The large terminase protein is a key component of the DNA packaging machinery in tailed bacteriophages and evolutionarily related herpes viruses. Typically, in addition to an ATPase domain which powers DNA translocation, the large terminase contains a nuclease domain which cuts concatemeric DNA, generated by rolling circle replication. Crystal structures of the large terminase nuclease from the thermophilic bacteriophage G20c show that it is most similar to the RuvC family of the RNase H-like endonucleases. The overall structure adopts the RNase-H fold.

Structures for complexes with Mn2+, Mg2+, Co2+ and Ca2+ were determined by soaking crystals of the apo protein, whereas the structure of the Zn2+ complex was obtained by co-crystallization. Only one metal ion, bound to the site A, was identified for conditions containing Mg2+, Mn2+ and Co2+. This metal ion is coordinated by the side chains of D294 and D429 and four water molecules in the canonical octahedral geometry. The nuclease was active in the presence of Mn2+, Mg2+ and Co2+ but inactive with Ni2+, Zn2+ or Ca2+, consistent with observations for T4 gp17 (41), SPP1 G2P and HCMV UL89 (18). However, G20c nuclease had minimal activity with Co2+, in contrast to the high non-specific in vitro nuclease activity observed for SPP1 G2P nuclease (comparable with Mn2+ (39)) or the absence of activity for the T4 gp17 nuclease.

>[2x]GPAMNSVFSGLDMLILLPYERRGTRLVVEDYRPDHIYCIGADFGKNQDYSVFSVLDLDTGAIACLERMNGATWSDQVARLKALSEDYGHAYVVADTWGVGDAIAEELDAQGINYTPLPVKSSSVKEQLISNLALLMEKGQVAVPNDKTILDELRNFRYYRTASGNQVMRAYGRGHDDIVMSLALAYSQYEG3-[(2Z)-3-methylpent-2-en-1-yl]benzene-1,2-diol | C12 H16 O2 | 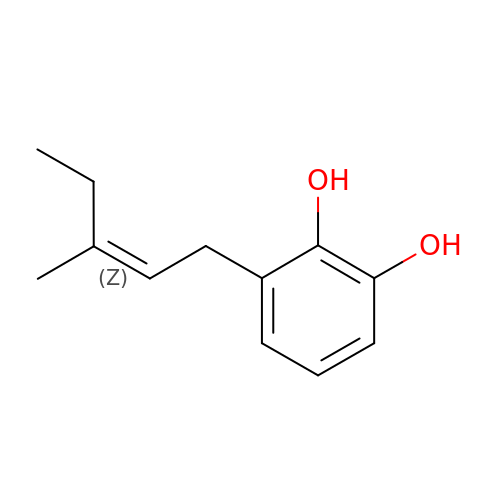HZIMMWSOLFBHHZ-CLFYSBASSA-N>[3x]GPAMKKLKPAPFYFQPFSKKQLKVLTWWRKASPVSDKDGIICDGSIRAGKTIVMSFSYVMWAMDTFNEQNFGMAGKTIGALRRNVITPLKRMLKSRGYRVKDHRADNYLTITFKGKTNYFYLFGGKDESSQDLIQGITLAGMFFDEVALMPESFVNQATARCSV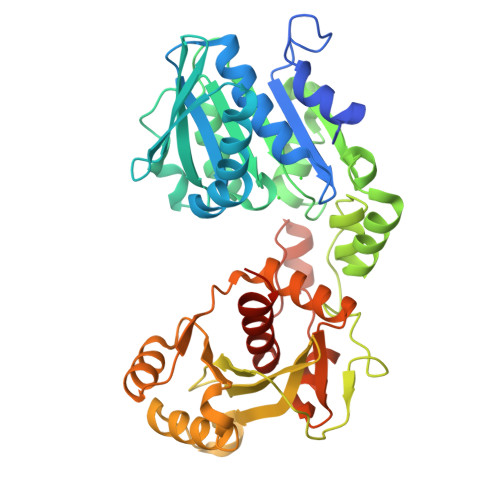DGAKLWFNCNPAGPYHWFKVEYLDKLDEKNLLHLHFTMDDNLSLSKQVKERYQRMYKGVFYQRYILGLWVLAEGIIYDMFDQDEHVVPTVPRPYEKYYVSCDYGTQNPTTFGLWGLYNGVWYKVKEYHYDGRKENKQKTDQEYYEDLMKFIEDIEKHKFKGVIVDPSAASFIALLRQKGIKVIKAKNDVLDGIRNVATALNKKMILYNDCCKETFREYSSYVWDEKAAERGEDKPVKQNDHQLDADRYFVNTILFGNKLRAVPSLY>[4x]MGWSLPKEKGLILCLWNKFCRWFHRRESWAQSRDEQNLLQQKRIWESPLLLAAKENNVQALYKLLKFEGCEVHQKGAMGETALHIAALYDNNEAAQVLMEAAPELVFEPMTSELYEGQTALHIAVINQNVNLVRALLARGASVSARATGSVFHYRPHNLIYYGEHPLSFAACVGSEEIVRLLIEHGADIRAQDSLGNTVLHILILQPNKTFACQMYNLLLSYDGGDHLKSLELVPNNQGLTPFKLAGVEGNIVMFQHLMQKRKHIQWTYGPLTSTLYDLTEIDSSGDDQSLLELIVTTKKREARQILD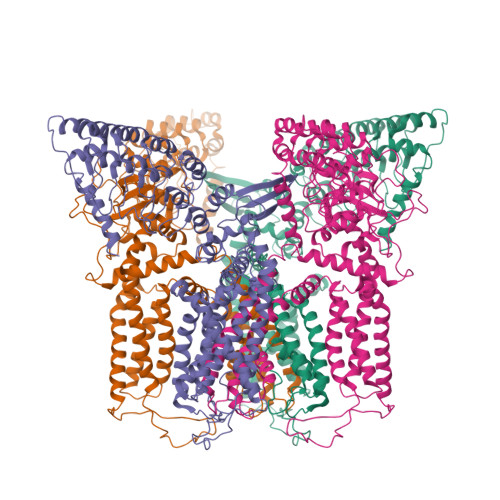QTPVKELVSLKWKRYGRPYFCVLGAIYVLYIICFTMCCVYRPLKPRITNRTNPRDNTLLQQKLLQEAYVTPKDDLRLVGELVSIVGAVIILLVEIPDIFRLGVTRFFGQTILGGPFHVIIVTYAFMVLVTMVMRLTNSDGEVVPMSFALVLGWCNVMYFARGFQMLGPFTIMIQKMIFGDLMRFCWLMAVVILGFASAFYIIFQTEDPDELGHFYDYPMALFSTFELFLTIIDGPANYDVDLPFMYSITYAAFAIIATLLMLNLLIAMMGDTHWRVAHERDELWRAQVVATTVMLERKLPRCLWPRSGICGREYGLGDRWFLRVEDRQDLNRQRIRRYAQAFQQQDDLYSEDLEKDSGEKLVPR> AAAAAAAAAAAAAAAAAAAAAAAAAAAAAAAAAAAAAAAAAAAAAAAAAAAAAAAAAAAAAAAA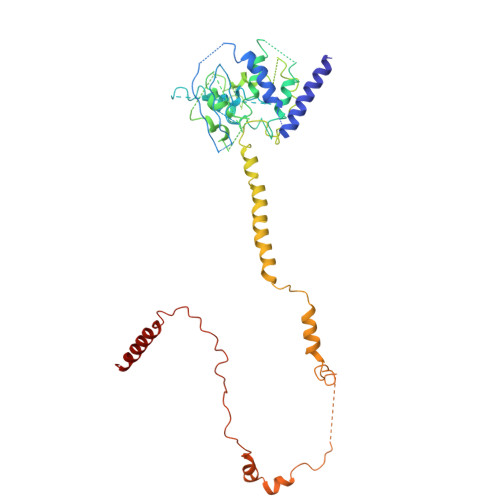AAAAAAAAAAAAAAAAAAAAAAAAAAAAAAAAAAAAAAAAAAAAAAAAAAAAAAAAAAAAAAAAAAAAAAAAAAAAAAAAAAAAAAAAAAAAAAAAAAAAAAAAAAAAAAAAAAAAAAAAAAAAAAAAAAAAAAAAAAAAAAAAAAAAAAAAAAAAAAAAAAAAAAAAAAAAAAAAAAAAAAAAAAAAAAAAAAAAAAAAAAAAARAAAAAAAAAAAAAAAAAAAAAAAAAAAAAAAAAAAAAAAAAAAAAAATTKEAYKKLSQKFHGTKSNKK>[2x]MGGSHHHHHHGMASLAPGSSRVELFKRQSSKVPFEKDGKVTERVVHSFRLPALVNVDGVMVAIADARYETSFDNSLIDTVAKYSVDDGETWETQIAIKNSRASSVSRVVDPTVIVKGNKLYVLVGSYNSSRSYWTSHGDARDWDILLAVGEVTKSTAGGKITASIKWGSPVSLKEFFPAEMEGMHTNQFLGGAGVAIVASNGNLVYPVQVTNKKKQVFSKIFYSEDEGKTWKFGKGRSAFGCSEPVALEWEGKLIINTRVDYRRRLVYESSDMGNTWLEAVGTLSRVWGPSPKSNQPGSQSSFTAVTIEGMRVMLFTHP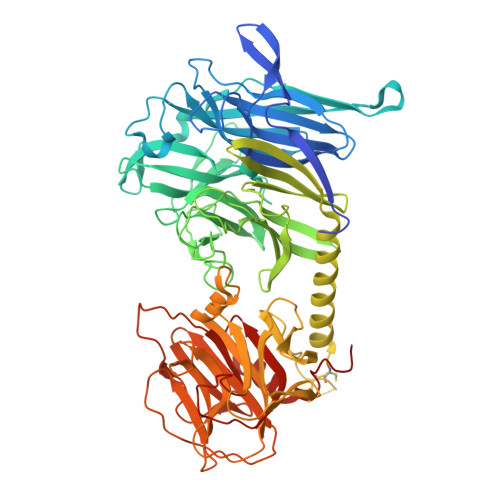LNFKGRWLRDRLNLWLTDNQRIYNVGQVSIGDENSAYSSVLYKDDKLYCLHEINSNEVYSLVFARLVGELRIIKSVLQSWKNWDSHLSSICTPADPAASSSERGCGPAVTTVGLVGFLSHSATKTEWEDAYRCVNASTANAERVPNGLKFAGVGGGALWPVSQQGQNQRYFFANHAFTLVASVTIHEVPKGASPLLGASLDSSGGKKLLGLSYDKRHQWQPIYGSTPVTPTGSWEMGKRYHVVLTMANKIGSVYIDGEPLEGSGQTVVPDERTPDISHFYVGGYKRSGMPTDSRVTVNNVLLYNRQLNAEEIRTLFLSQDLIGTEAHMD>PYNKIVSHLLVAEPEKIYAMPDPTVPDSDIKALTTLCDLADRELVVIIGWAKHIPGFSTLSLADQMSLLQSAWMEILILGVVYRSLSFEDELVYADDYIMDEDQSKLAGLLDLNNAILQLVKKYKSMKLEKEEFVTLKAIALANS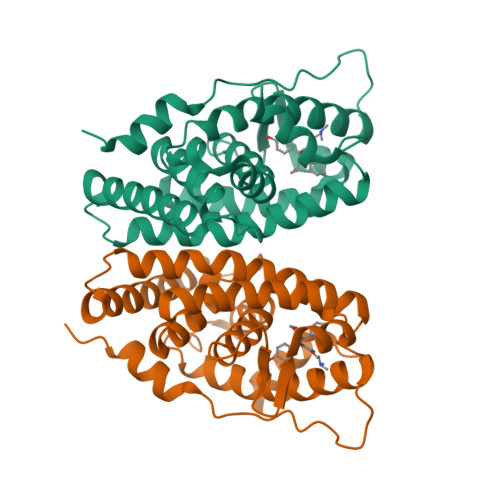DSMHIEDVEAVQKLQDVLHEALQDYEAGQHMEDPRRAGKMLMTLPLLRQTSTKAVQHFYNIKLEGKVPMHKLFLEMLEAKV[5x]> VLGKPQTDPTLEWFLSHCHIHKYPSKSTLIHQGEKAETLYYIVKGSVAVLIKDEEGKEMILSYLNQGDFIGELGLFEEGQERSAWVRAKTACEVAEISYKKFRQLIQVNPDILMRLSAQMARRLQVTSEKVGNLAFLDVTGRIAQTLLNLAKQPDAMTHPDGMQIKITR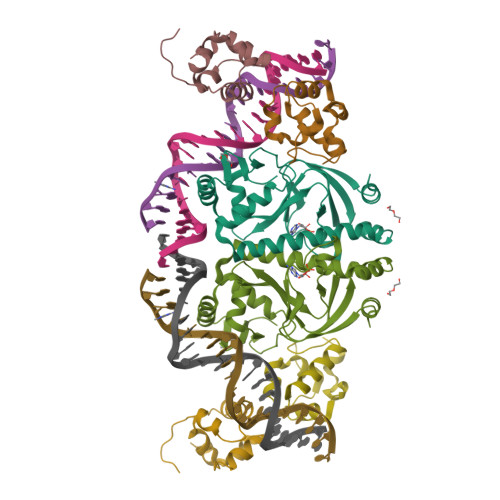QEIGQIVGCSRETVGRILKMLEDQNLISAHGKTIVVYGTR;>[2x]KPEFDPILLRPVDDLELTVRSANCLKAEAIHYIGDLVQRTEVELLKTPNLGKKSLTEIKDVLASRGLSLGMRLENWPPASIADE>[2x]GHMLSKRDAILKAAVEVFGKKGYDRATTDEIAEKAGVAKGLIFHYFKNKEELYYQAYMSVTEKLQKEFENFL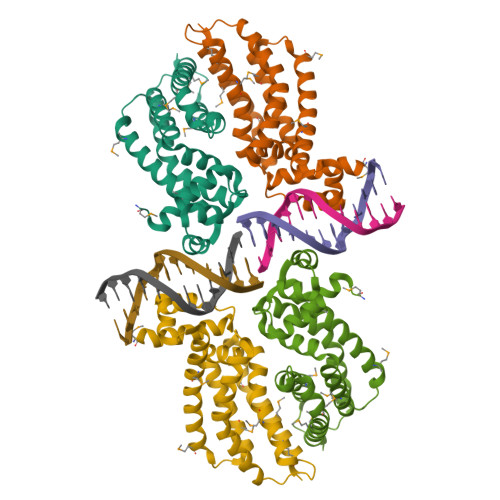MKNRNRDIFDFMERWIEKKLEYSASHPEEADFLITLVSVDEGLRKRILLDLEKSQRVFFDFVREKLKDLDLAEDVTEEIALKFLMWFFSGFEEVYLRTYQGKPELLKRDMNTLVEEVKVMLRILKKGMTK>MKHLEEKTLSTRQIFKGRYLKIEQDQVQAPDGRTYTREYILHPGAAMMIPLLPNGNVVMIHQYRHAVKKVFLEFPAGKRDHNEETLLTAKRELLEETGYEAKDWKFLTTIHPVIGYSNEHIDLYLARDLTHLEQRLDQGQFIEVVEVKPADLMQLVLEGKVSDVKTQIGAFWLDK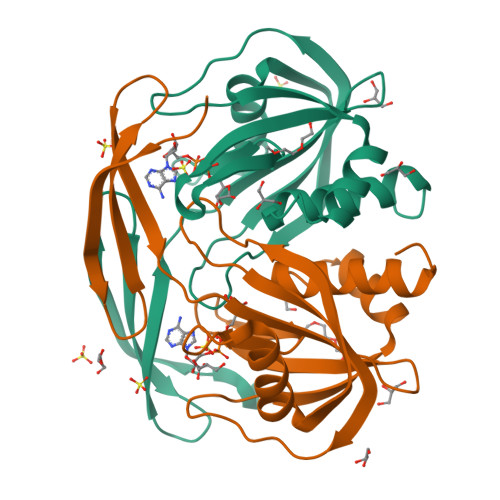FLRGEWN[2x]> TIQPGTGYNNGYFYSYWNDGHGGVTYTNGPGGQFSVNWSNSGEFVGGKGWQPGTKNKVINFSGSYNPNGNSYLSVYGWSRNPLIEYYIVENFGTYNPSTGATKLGEVTSDGSVYDIYRTQRVNQPSIIGTATFYQYWSVRR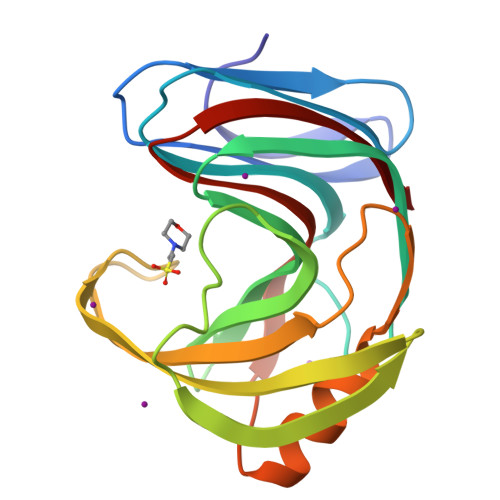NHRSSGSVNTANHFNAWAQQGLTLGTMDYQIVAVEGYFSSGSASITVS>ACPAPPPGQPDIRAIGYYTDKAGSVIDPALQQQNKDATAPLDRYAADVARMSDDYLRNGDPAAAQCTLSWLGAWADDGAMLGQMIRVNNDQSFYMRQWMLDAVAMAYLKVHDQANPQQRARIDPWLQKLARANLAYWDNPKRRRNNHYYWGGLGVLATGLATDDDALWQAGHAAFQKGIDDIQDDGSLPLEMARGQRALHYHDYALAPLVMMAELARLRGQDWYASRNHAIDRLARRVIEGSRDPAWFNQHTGAAQL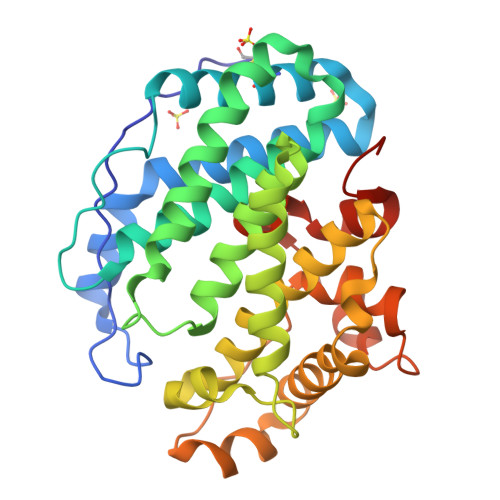PLQASGWVEFYRLRSPDGGVFDAAHARGPFHSPRLGGDLTLMATHGIVRTPLRHHHHHH[2x]ETHIDIUM | C21 H20 N3 | 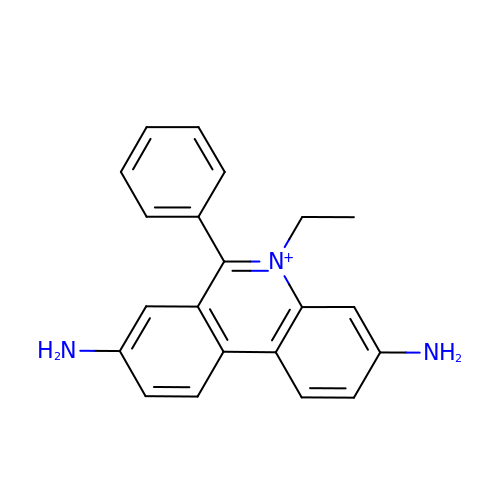QTANTQQOYSUMLC-UHFFFAOYSA-O>GSASKICQFKLVLLGESAVGKSSLVLRFVKGQFHEYQESTIGAAFLTQSVCLDDTTVKFEIWDTAGQERYHSLAPMYYRGAQAAIVVYDITNQETFARAKTWVKELQRQASPSIVIALAGNKADLANKRMVEYEEAQAYADDNSLLFMETSAKTAMNVNDLFLAIAKKLPKSEPQNLGG[2x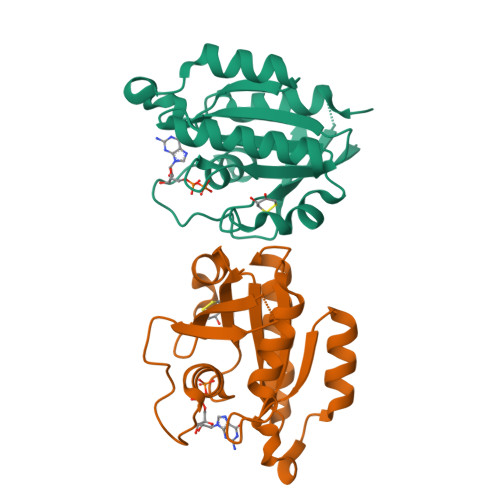]>MSNIQNMSLEDIMGERFGRYSKYIIQDRALPDIRDGLKPVQRRILYSMNKDSNTFDKSYRKSAKSVGNIMGNFHPHGDSSIYDAMVRMSQNWKNREILVEMHGNNGSMDGDPPAAMRYTEARLSEIAGYLLQDIEKKTVPFAWNFDDTEKEPTVLPAAFPNLLVNGSTGISAGYATDIPPHNLAEVIDAAVYMIDHPTAKIDKLMEFLPGPDFPTGAIIQGRDEIKKAYETGKGRVVVRSKTEIEKLKGGKEQIVITEIPYEINKANLVKKIDDVRVNNKVAGIAEVR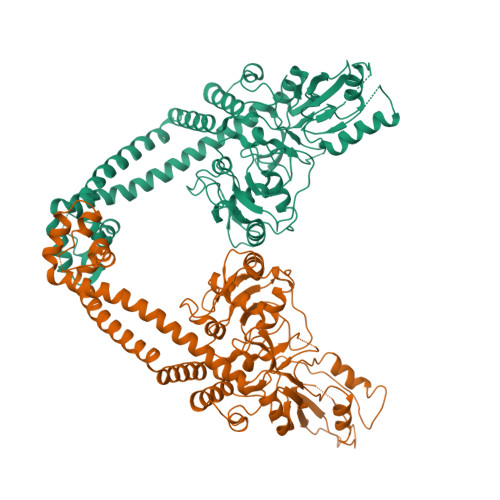DESDRDGLRIAIELKKDANTELVLNYLFKYTDLQINYNFNMVAIDNFTPRQVGIVPILSSYIAHRREVILARSRFDKEKAEKRLHIVEGLIRVISILDEVIALIRASENKADAKENLKVSYDFTEEQAEAIVTLQLYRLTNTDVVVLQEEEAELREKIAMLAAIIGDERTMYNLMKKELREVKKKFATPRLSSLEDTAKALEHHHHHH[4x]>[2x]MRPNLLAAAIAVPLSLLAAQIAQAGEGMWVPQQLPEIAGPLKKAGLKLSPQQISDLTGDPMGAVVALGGCTASFVSPNGLVVTNHHCAYGAIQLNSTAENNLIKNGFNAPTTADEVSAGPNARVFVLDEITDVTKDAKAAIAAAGDDALARTKALEAFEKKLIADCEAEAGFRCRLYSFSGGNTYRLFKNLEIKDVRLAYAPPGSVGKFGGDIDNWMWPRHTGDFAFYRAYVGKDGKPAAFSKDNVPYQPKHWLKFADQPLGAGDFVMVAGYPGSTNRYALAAEFDNTAQWTYPTIARHYKNQIAMVEAAGKQNADIQVKYAATMAGWNNTSKNYDGQLEGFKRIDAAGQKLREEAAV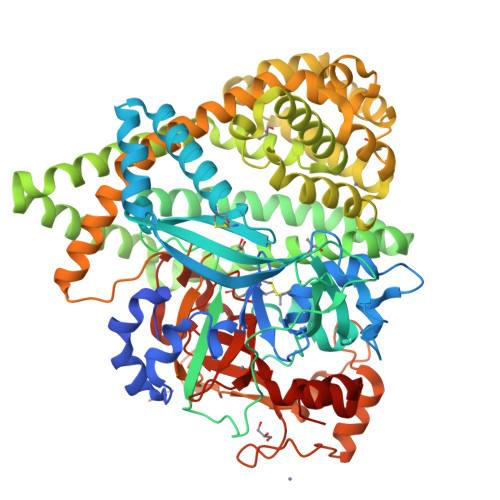LGWLKGQGAKGQPALDAHAKLLDLLEQSKATRDRDLTLALFNNTAMLGSATQLYRLSIEREKPNAERESGYQERDLPAIEGGLKQLERRYVAAMDRQLQEYWLNEYIKLPADQRVAAVDAWLGGNDAAAVKRALDRLAGTKLGSTEERLKWFAADRKAFEASNDPAIQYAVAVMPTLLKLEQERKTRAGENLAARPVYLQALADYKKSQGEFVYPDANLSLRITFGNVMGYAPKDGMEYTPFTTLEGVVAKETGQDPFDSPKALLDAVAAKRYGGLEDKRIGSVPVNYLSDLDITGGNSGSPVLDAHGKLVGLAFDRNWESVSSNWVFDPKMTRMIAVDGRYLRWIMQEVYPAPQLLKEMNVGK> AAAAAMTMMDMNFKYCHKIMKKHSKSFSYAFDLLPEDQRKAVWAIYAVCRKIDDSIDVYGDIQFLNQIKEDIQSIEKYPYEYHHFQSDRRIMMALQHVAQHKNIAFQSFYNLIDTVYKDQHFTMFETDAELFGYCYGVAGTVGEVLTPILSDHETHQTYDVARRLGESLQLINILRDVGEDFENERIYFSKQRLKQYEVDIAEVYQNGVNNHYIDLWEYYAAIAEKDFRDVMDQIKVFSIEAQPIIELAARIYIEILDEVRQANYTLHERVFVEKRKKA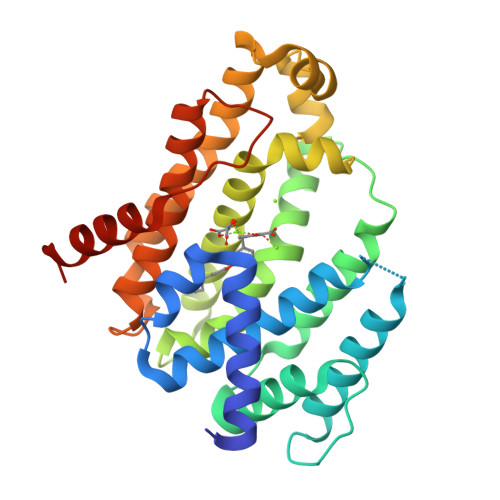KLFHEINSKYHRI>[2x]MSLDNLDVICIGAAIVDIPLQPVSKNIFDVDSYPLERIAMTTGGDAI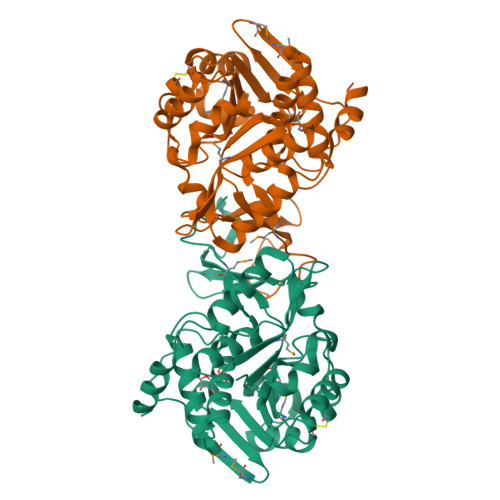NEATIISRLGHRTALMSRIGKDAAGQFILDHCRKENIDIQSLKQDVSIDTSINVGLVTEDGERTFVTNRNGSLWKLNIDDVDFARFSQAKLLSLASIFNSPLLDGKALTEIFTQAKARQMIICADMIKPRLNETLDDICEALSYVDYLFPNFAEAKLLTGKETLDEIADCFLACGVKTVVIKTGKDGCFIKRGDMTMKVPAVAGITAIDTIGAGDNFASGFIAALLEGKNLRECARFANATAAISVLSVGATTGVKNRKLVEQLLEEYEGEGHHHHHH>[4x]MPLILLPAVDVVEGRAVRLVQGKAGSQTEYGSAVDAALGWQRDGAEWIHLVDLDAAFGRGSNHELLAEVVGKLDVQVEL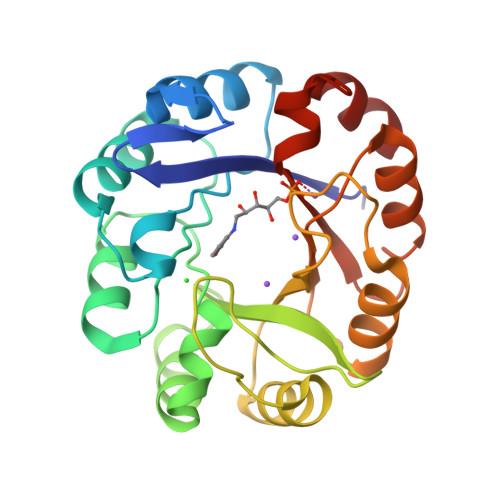SGGIRDDESLAAALATGCARVNVGTAALENPQWCARVIGEHGDQVAVGLDVQIIDGEHRLRGRGWETDGGDLWDVLERLDSEGCSRFVVTDITKDGTLGGPNLDLLAGVADRTDAPVIASGGVSSLDDLRAIATLTHRGVEGAIVGKALYARRFTLPQALAAVRD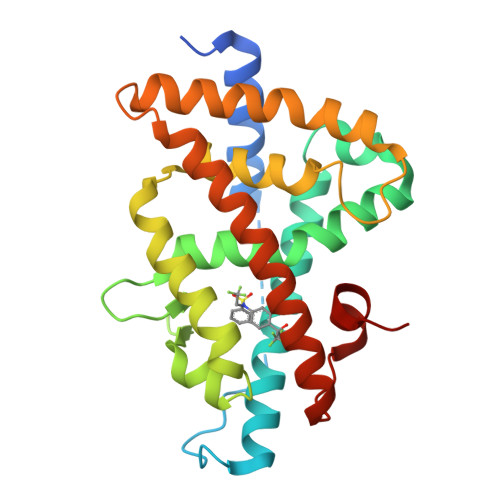> GSHMSQGSGEGEGVQLTAAQELMIQQLVAAQLQCNKRSFSDQPKVTPWPLGADPQSRDARQQRFAHFTELAIISVQEIVDFAKQVPGFLQLGREDQIALLKASTIEIMLLETARRYNHETECITFLKDFTYSKDDFHRAGLQVEFINPIFEFSRAMRRLGLDDAEYALLIAINIFSADRPNVQEPGRVEALQQPYVEALLSYTRIKRPQDQLRFPRMLMKLVSLRTLSSVHSEQVFALRLQDKKLPPLLSEIWDVHE>[3x]SNAMKAIITVVGKDKSGIVAG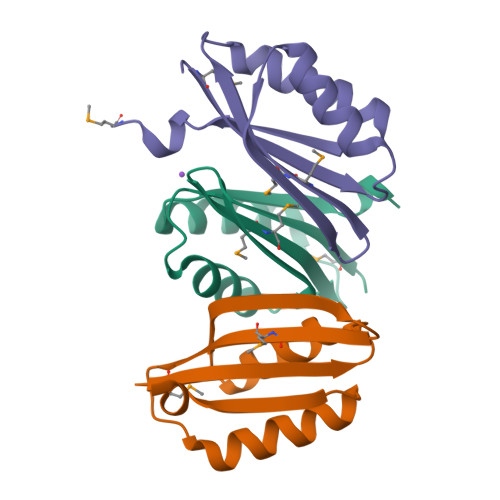VSGKIAELGLNIDDISQTVLDEYFTMMAVVSSDEKQDFTYLRNEFEAFGQTLNVKINIQSAAIFEAMYNI(3R)-4-[6-{1-[diamino(hydroxy)-lambda~4~-sulfanyl]cyclopropyl}-2-(methylsulfanyl)pyrimidin-4-yl]-3-methylmorpholine 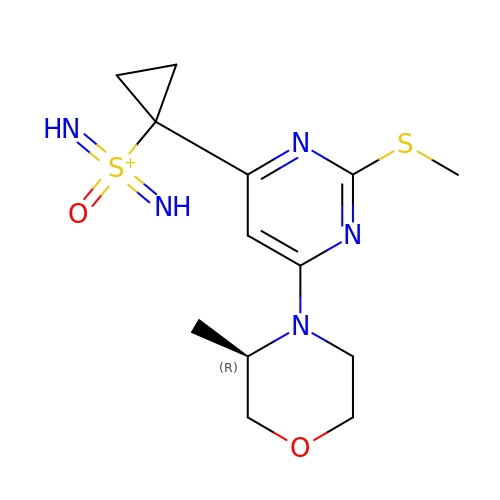| C13 H20 N5 O2 S2 | IBTBNJWCWMILQN-SECBINFHSA-N> MDCSTGAAIGQQFAKDAFHMHGGVGVGPTGNSEHDVLMNEMMMVQTPTGPAGEWTHQFAAYQGQQQQQQQQHPQELAMRHQQNDAFMLRQQQEMEEAFCTFCTTHPHSHAHSHQPQGLVGPAMMGPQIMPPMMFGPGTGGFMMGAPPMMPYASMKFAGDAAMAAANNTNMTQGATATSTTSVQQELQQQSSDNGWVEKLRDAEWAQDYSDAQVFTLEGQSEQTMEEHAKNSEFYQFMDKIRSKELLIDEETGQLVQGPGPDPDAPEDAEYLKEWAAAEGLNMPPGFFEHMMQRPQGNNEQAEGRLFDGSNDALMDDGALDNAADVEEWVREYAEAQEQLQRVQNETNYPFEPNNPYMYHDKPMEEGIAMLQLANMAEAALAFEAVCQKEPENVEAWRRLGTTQAENEKDCLAIIALNHARMLDPKDIAVHAALAVSHTNEHNVGAALQSLRSWLLSQPQYEHLGLVDLREVAADEGLDEVPEENYFFAAPSEYRDCCTLLYAAVEMNPNDPQLHASLGVLHNLSHRFDEAAKNFRRAVELRPDDAHMWNKLGATLANG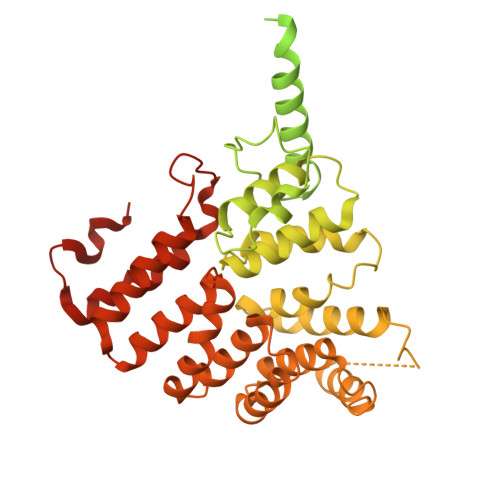NRPQEALEAYNRALDINPGYVRVMYNMAVSYSNMAQYPLAAKHITRAIALQAGGTNPQGEGSRIATRGLWDLLRMTLNLMDRSDLVEASWQQDLTPFLREFGLEEMAV1-O-phosphono-alpha-D-mannopyranose | C6 H13 O9 P | 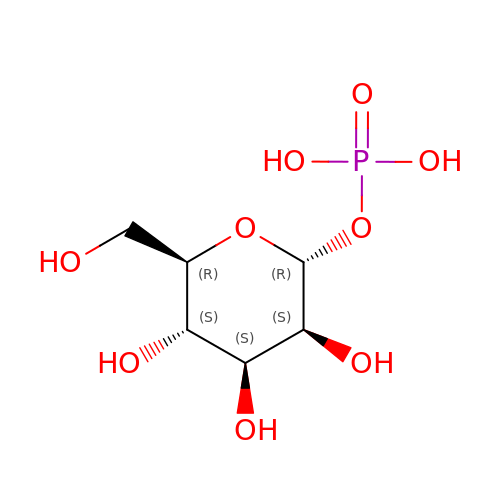HXXFSFRBOHSIMQ-RWOPYEJCSA-N> MRCVGIGNRDFVEGLSGATWVDVVLEHGS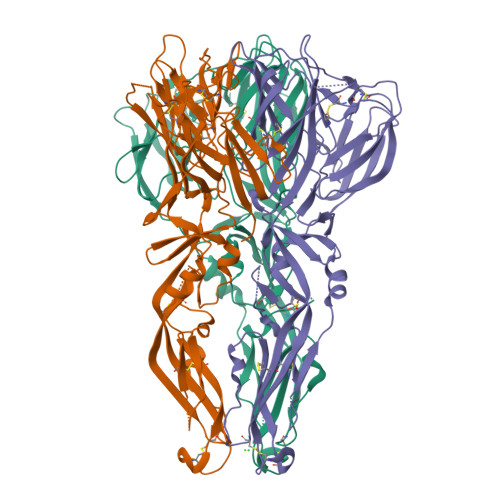CVTTMAKDKPTLDIELLKTEVTNPAVLRKLCIEAKISNTTTDSRCPTQGEATLVEEQDANFVCRRTFVDRGWGNGCGLFGKGSLLTCAKFKCVTKLEGKIVQYENLKYSVIVTVHTGDQHQVGNETTEHGTIATITPQAPTSEIQLTDYGALTLDCSPRTGLDFNEMVLLTMKEKSWLVHKQWFLDLPLPWTSGASTSQETWNRQDLLVTFKTAHAKKQEAVVLGSQEGAMHTALTGATEIQTSGTTTIFAGHLKCRLKMDKLTLKGISYVMCTGSFKLEKEVAETQHGTVLVQVKYEGTDAPCKIPFSSQDEKGVTQNGRLVTANPIVTDKEKPVNIEAEPPFGESYIVVGAGEKALKLSWFKKGSSIGK2-[2-[[3-[(3~{S})-3-azanyl-2,3-dihydro-1-benzofuran-5-yl]-5-(2-cyanopropan-2-yl)phenyl]methoxy]phenyl]ethanoic 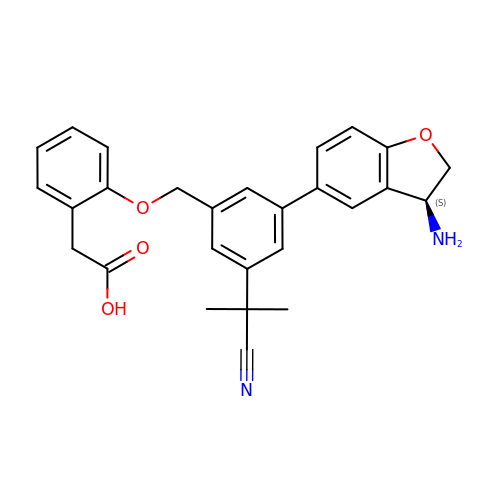acid | C27 H26 N2 O4 | SRKDCGUSWAONMJ-HSZRJFAPSA-N>SMLTELIASNRRSAAIHAFVDTGLSTHFKDGIYVDISELSRKSGVNYARFSRLCDFLVEMGVLVSNDNKFRLSDECHVFANPESFESFMIKLEICSHYSNAWLMYGKSLFEDDGKSAFEMAHGRPFFEYLDGNKFLKSNFDALMTRVSNLIVEKLLGIYDFNQHNRILDVGGGEGELLVRISEKVKGKHYAVLDRYSELPVSDNIDFINGNFLNSIPSGYDLYILKNVLHNWSDSDSILILENFRKAMDKNSSLLLINMVKEPEFSRS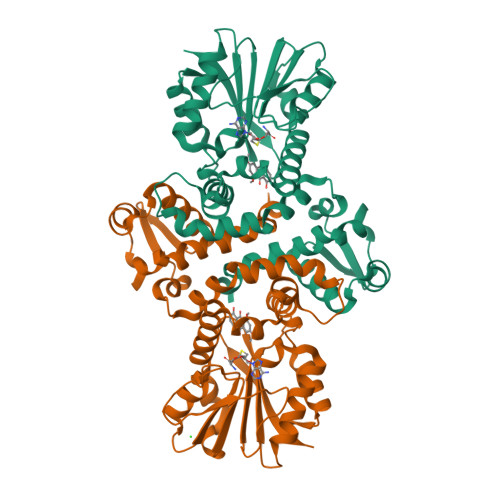FDILMDVLFLGKERSFTEFEYLANQAGLVVQETKVIDQSYSPYSFIKLQIK[4x]>[2x]SNAMEKPDPKVIVAIDAGTVEQARAQ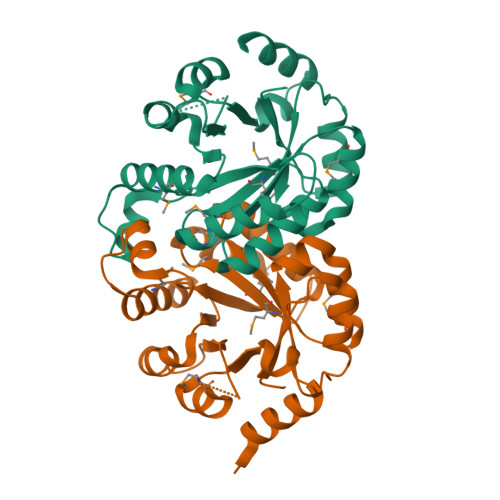INPLTPELCHLKIGSILFTRYGPAFVEELMQKGYRIFLDLKFYDIPQTVAGACRAVAELGVWMMNIHISGGRTMMETVVNALQSITLKEKPLLIGVTILTSLDGSDLKTLGIQEKVPDIVCRMATLAKSAGLDGVVCSAQEAALLRKQFDRNFLLVTPGIRLETDEKGDQKRVMTPRAAIQAGSDYLVIGRPITQSTDPLKALEAIDKDIKTR> MSKQFVRSAKNLVKGYSSTQVLVRNATSNDNHQVSKDSLIELAEKSYDSADFFEIMDMLDKRLNDKGKYWRHIAKALTVIDYLIRFGSENCVLWCRENLYIIKTLKEFRHEDDEGIDQGQIVRVKAKELTALLSDDERLNEERNMNIKGRN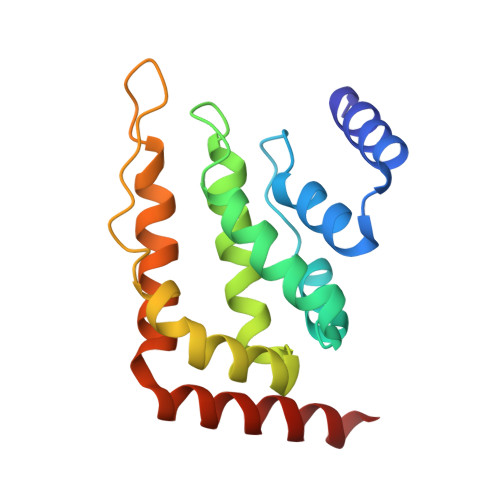RKG> GKKSRMCGYCGAPAPYATACGLDVCVYHTHFHQHCPVIIWCGHPAGSGSCSECEPPLGKGTSPLDEVLEQVPYKPPRTVIMHVEQGLTPLDPGRYQTRRGLVSVRRGIRGNEVDLPDGDYASTALLPTCKEINMVAVASNVLRSRFIIGPPGAGKTHWLLQQVQDGDVIYTPTHQTMLDMIRALGTCRFNVPAGTTLQFPAPSRTGPWVRILAGGWCPGKNSFLDEAAYCNHLDVLRLLSKTTLTCLGDFKQLHPVGFDSHCYVFDIMPQTQLKTIWRFGQNICDAIQPDYRD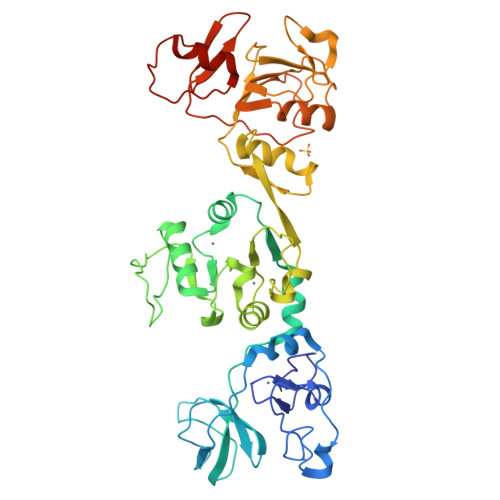KLMSMVNTTRVTYVEKPVRYGQVLTPYHRDREDSAITIDSSQGATFDVVTLHLPTKDSLNRQRALVAITRARHAIFVYDPHRQLQSVFDLPAKGTPVNLAVHRDEQLIVLDRNNREITVAQALGNGDKFRATDKRVVDSLRAICADLE>VEKNITVTASVDPAIDLLQADGNALPSAVKLAYSPASKTFESYRVMTQVHTNDATKKVIVKLADTPQLTDVLNSTVQMPISVSWGGQVLSTTAKEFEAAALGYSASGVNGVSSSQELVISAAPKTAGTAPT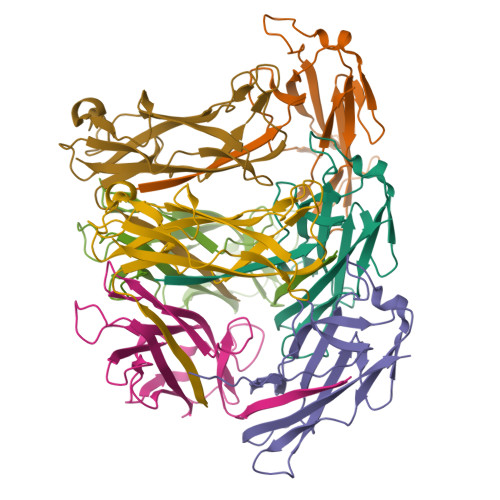AGNYSGVVSLVMTLG[7x]> MIFAVRTMVGQEKNIAGLMASRAEKEQLDVYSILASESLKGYVLVEAETKGDVEELIKGMPRVRGIVPGTIAIEEIEPLLTPKKIIENIEKGDVV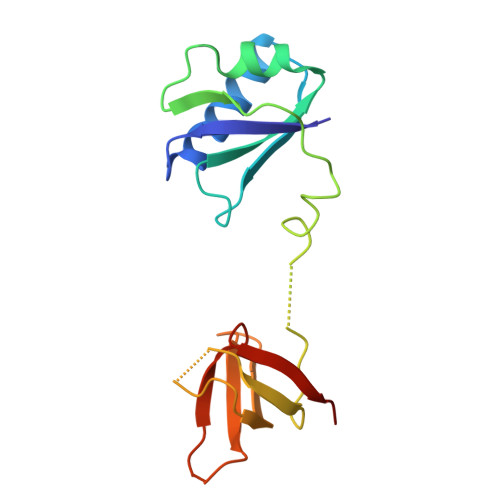EIIAGPFKGERAKVIRVDKHKEEVTLELENAAVPIPITLPVEGVKIVSKHKD We have described herein the reactions and the structure of Pgp3, a Csd protein of C. jejuni. This enzyme turns over the cell-wall peptidoglycan by both the d,d-endopeptidase and d,d-carboxypeptidase activities, as documented by mass spectrometric characterization of the requisite reactions with synthetic cell-wall fragments. The Pgp3 monomer is structurally divided into four regions: the N-terminal domain (NTD, residues 21–95), a flexible linker (residues 96–147), the LytM domain (residues 148–259), and the C-terminal helix (residues 260–273). The Pgp3 LytM domain contains a highly conserved tetrahedral Zn2+-ion-binding motif (H168xxxD172 and HxH249).

In order to gain mechanistic insight into how Pgp3 works, we have determined the X-ray structures of the WT Pgp3 in two crystal forms (bound separately to tartrate and to citrate). For the tartrate-bound WT, a model accounting for all the amino acids of the recombinant Pgp3 (Glu21-Asn273) was refined at a resolution of 1.86 Å to Rwork and Rfree values of 17.2% and 19.9%, respectively. Crystals of Pgp3 could only be produced in the presence of either tartrate or citrate molecules. Both molecules bound to the active site of Pgp3 via several hydrogen bonds and salt-bridge interactions between the carboxyl groups of tartrate or citrate and the Zn2+ ion. Furthermore, in the tartrate-bound complex, the side chain of His216 (NE2 atom) formed a hydrogen bond with the O3 of the tartrate molecule (3.4 Å), and the side chain of His247 (NE2 atom) formed another hydrogen bond with tartrate O3 atom (2.7 Å). The O3 atom of tartrate in WT Pgp3 (open form), which is the position of Wat-1 in H247A variant, is seen interacting with His216 and His247. Specifically, in the tartrate-bound complex, Wat-1 and Wat-2 were displaced by tartrate O3 and O41 atoms, and in the citrate-bound WT Pgp3, they were displaced by citrate O5 and O6 atoms, respectively. When the structure of Pgp3 in complex with tartrate was overlaid with that of the citrate complex, their overall structures were similar with RMSD of 2.95 Å over 256 equivalent Cα positions. However, both structures showed a large deviation (RMSD 6.98 Å) in two regions (residues Glu99-Phe109 and Thr159-Val164) near the active-site.

> MELIKGQALFLELDKKDFLSLKNNDKNIPTFAHPKNQEKILAIFSLPYKNPPQNTKLIAFYKDKKEEIFIKTLEGNYKSEKLQVENKKIFPPKTIQERIAKELKEANAIYSSYTPKALFNGAFNIPLNSFITSDFGKARTFNEKVASYHSGTDFRAATGTPIYAANSGVVKIAKDRYFAGNSVVIDHGFGIYSQYYHLSKIDVKVGQKIKKGELIGLSGASGRVSGPHLHFGILAGGKQVDPLDFVSKFNAIFQLEHHHHHH>[2x]MKKIEVYTQPDCPPCVIVKEFLKHNNVAYEEFDVKKDAAARNRLLYDYDSYSTPTVVIDGEVVAGFQIEKLQQLLNIE

Thioredoxin (Trx) and glutaredoxin (Grx) are small ubiquitous proteins acting as cysteine disulfide oxidoreductases in the cell and belong to the thioredoxin superfamily. The thioredoxin BC3987 found in B. cereus ATCC 14579 is conserved among all the members of the B. cereus group, including B. anthracis, B. mycoides, B. pseudomycoides, B. thuringiensis and B. weihenstephanensis. Like E. coli and C. ammoniagenes NrdH the BC3987 have a α/β/α Trx fold typical for all members of the Thioredoxin superfamily. The BC3987 protein has a C-P-P-C active site motif that differs from what is typically observed for Trxs and Grxs.

The crystal structure of oxidized BC3987 was solved and we have related the results from the phylogenetic analysis to structural features, enabling us to map parts of the protein involved in hydrogen bonds near the active site. The BC3987 wild type and T8A mutant structures were refined to 1.4 and 1.18 Å, respectively. In the wild type structure residues 1–76 and 3–75 are observed in chain A and B, respectively. Due to the insert of one Leu amino acid at position 44 in the BC3987 protein, the α2 helix is positioned slightly closer to the β-sheet layer compared to E. coli NrdH. Additionally, the residues Thr8 and Thr53 in the vicinity of the disulfide bridge are possible hydrogen bond partners for the buried C-terminal cysteine. Contrary to what is seen in the NrdH-redoxins from E. coli and C. ammoniagenes crystal structures the Thr8 residue in BC3987 has a rotamer where the hydroxyl group is pointing away from the buried Cys15 Sγ-atom. This orientation of Thr8 is stabilized by a hydrogen bond to a water molecule (HOH34). The proline residues apply restrictions on the protein backbone, making a rigid frame for the active site cysteines. Both proline residues in the BC3987 active site have the trans-conformation with ω-angles of 177° and 176° for the Pro13 and Pro14, respectively.>[2x]GMENIPFLRASTVPVIEYLDELKEIDASHIYTNYGPINQRFEQTIMSGFFQNRGAVTTVANATLGLMAAIQLKKRKKGKYALMPSFTFPATPLAAIWCGLEPYFIDISIDDWYMDKTVLWDKIEELKEEVAIVVPYATFGSWMNLEEYEELEKKGVPVVVDAAPGFGLMNGGMHYGQ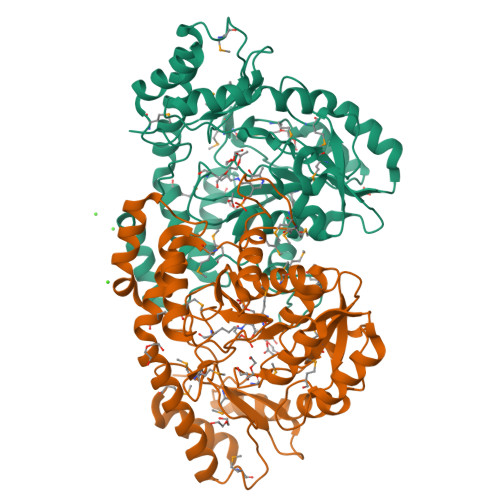DFSGMIIYSFHATKPFGIGEGGLIYSKNEEDIQRIKRMGNFGFDTNRECTMMGFNCKMSEYAAAIGIATMKKWDDKLKERTRISEWYKQLLQSNGLMKKGWQLQKTEAVIQQFMPILCPEEVRNKQVIEDLKKQKIEARLYFSPSCHQQVLFRNYKSTDLTRTNKIAKRIVSLPLWEGMTKEIVEQIVICLGQKVVSADE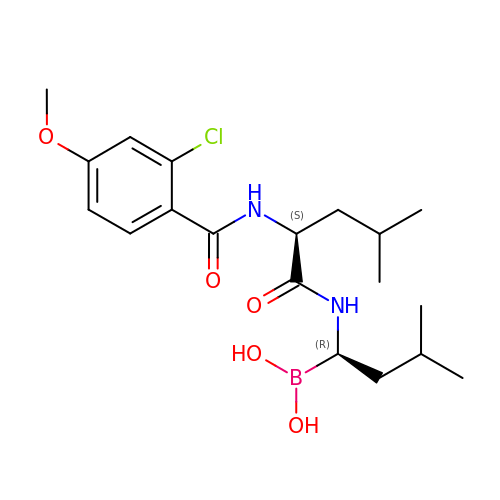N-[(1R)-1-borono-3-methylbutyl]-N~2~-(2-chloro-4-methoxybenzene-1-carbonyl)-L-leucinamide | C19 H30 B Cl N2 O5 | IUZAVACFOSUDSF-IRXDYDNUSA-N> GSHMSAPLPLDELRTFAEVLDRVKAAYVEPVDDKTLLENAIKGMLSNLDPHSAYLGPEDFAELQESTSGEFGGLGIEVGSEDGFIKVVSPIDDTPAARAGIQPGDLIVQIDGKPTKGQSMTEAVDSMRGKAGSPITLTIVRDGGRPFDVELKRAIIKVKSVKSQVLEPGYAYLRITQFQVNTGEEVVKALNQLRKDNKGRLKGLVLDLRNNPGGVLQSAVEVADAFLTKGLIVYTKGRIANSELRFSADPADPSDKVPLVVLINGGSAAAAEIVAGA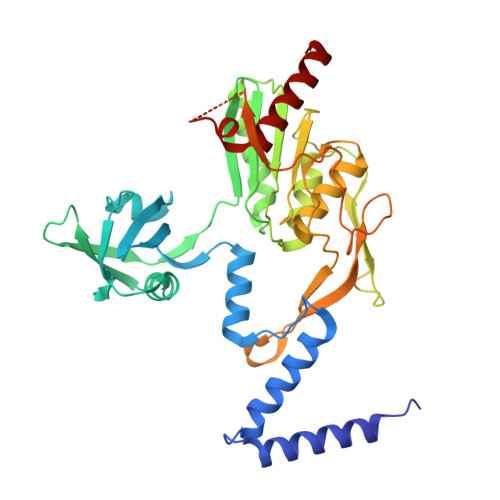LQDQKRAILMGTDSFGKGSVQTVLPLNNDRALKLTTALYYTPNGRSIQAQGIVPDIEVGRAKVTQERSSFEGFKEADLQGHLANGNGGADRPTGKRAAPSERPQDSDYQLSQALSLLKGLSVTRGN> G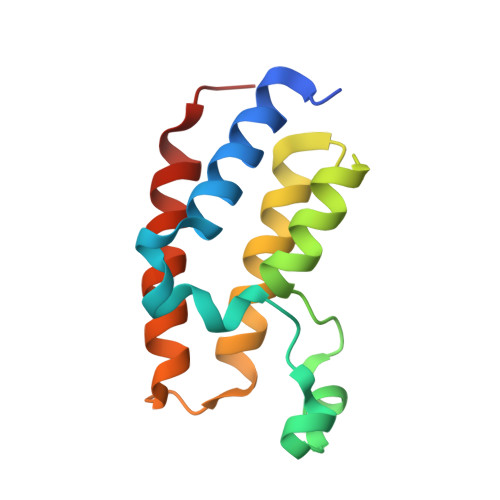PLGSKLSEHLRYCDSILREMLSKKHAAYAWPFYKPVDAEALELHDYHDIIKHPMDLSTVKRKMDGREYPDAQGFAADVRLMFSNCYKYNPPDHEVVAMARKLQDVFEMRFAKMPDEP> GPLGSARRLYVGNIPFGITEEAMMD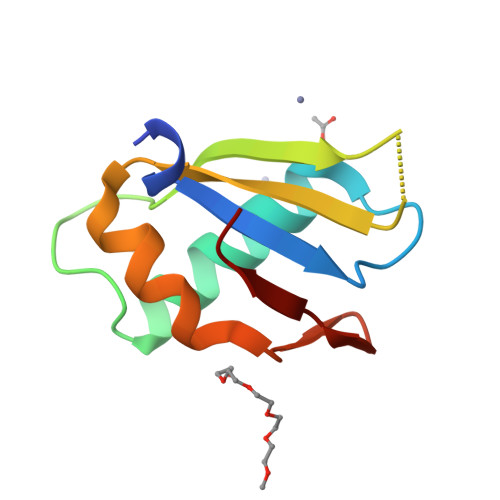FFNAQMRLGGLTQAPGNPVLAVQINQDKNFAFLEFRSVDETTQAMAFDGIIFQGQSLKIRRP>[2x]MHHHHHHHHHHSSGVDLGTENLYFQSNAMKTLEKVNYKGFIWPLAVGIVLWLITPWRPGGLSVQAWEMFAIFVATIVGCITKPLPIGGTTLLGMVVTVLVGLAPVKDVVNSKGVVIQTGILSSFGNSAAWLIAMAFIMAHGISKTGLGNRVAYVMIEKFGKRSIGIGYAITGLELMMGALIPSNSARTGGVTWPVVESISKSYDSKPNDPSRKKIGAYLDFMAFHANILSTALFITGAAPNLVAQQMAAQKGYQMSWVSWFWAALVPVLVATVIIPLVIYKMYPPEVKETPNAKNWADDKLKEMGPISKPEKIMATVFCLAILLWVLSGFFKIPQLDSAFVAFLAVTLLLITGVLSMEDALHETGAWNILIWLSILIFMAGKLISYGFIAWFAKFIQSEVHGINWGLVLVVLILLMFYTHYFFASGTAHMTALYLPFLTVATAMGAPLGLSAMLLAFTGVINASTTHYANGPASILATTGYVKQSEWWKMNFILGLIYMVIFGIVGTIWMKIIGIW

The mammalian SLC13 proteins are members of the larger divalent-anion sodium symporter (DASS) family. DASS proteins typically have a molecular weight of 45–65 kDa and form obligate homodimers. Each protomer consists of a scaffold and a transport domain. Structural information, along with cross-linking and computer modeling, indicates that DASS proteins operate in an elevator-type transport mechanism (Reyes et al., 2009; Drew and Boudker, 2016; Garaeva and Slotboom, 2020).

To obtain the structure of a DASS protein in its Co conformation, we screened various VcINDY homologs and chose a DASS-E protein from Lactobacillus acidophilus (LaINDY). Observing that the VcINDY structures were nearly identical in amphipol and nanodiscs, we surmised that amphipol was suitable for structure determination of another DASS protein, LaINDY. The LaINDY map obtained in this way was at 3.09 Å resolution, allowing for direct model building. The 3.09 Å cryo-EM map of LaINDY determined in the absence of substrate shows the transporter in its Co apo state. In agreement with LaINDY’s apparent mass in detergent solution, the map shows a transporter dimer. The transmembrane topology and domain organization of LaINDY resemble that of VcINDY, with the scaffold domain being formed by transmembrane α-helices TMs 1–4 and 7–9, while the transport domain consists of TMs 5, 6, 10 and 11, as well as the helix hairpins HPin and HPout. While LaINDY’s topology is similar to that of VcINDY, the relative domain positions are different. The transport domain is oriented toward the extracellular side with its substrate binding site facing the periplasm, yielding a Co conformation. Compared with VcINDY, the transport domain in LaINDY is repositioned by 13.0 Å towards the periplasm with a 37.4° rotation. All three Co-S structures are not only similar to each other but, importantly, also to the LaINDY Co apo structure, with pairwise r.m.s.d.s of 0.41–0.52 Å, indicating that substrate binding introduces little conformational change.> MEVNVKGNYVQVYVMLPLDAVSVNNRFEKGDELRAQLRKLVEAGVDGVMVDVWWGLVEGKGPKAYDWSAYKQLFELVQKAGLKLQAIMSFHQCGGNVGDAVNIPIPQWVRDVGTRDPDIFYTDGHGTRNIEYLTLGVDNQPLFHGRSAVQMYADYMTSFRENMKEFLDAGVIVDIEVGLGPAGEMRYPSYPQSHGWSFPGIGEFICYDKYLQADFKAAAAAVGH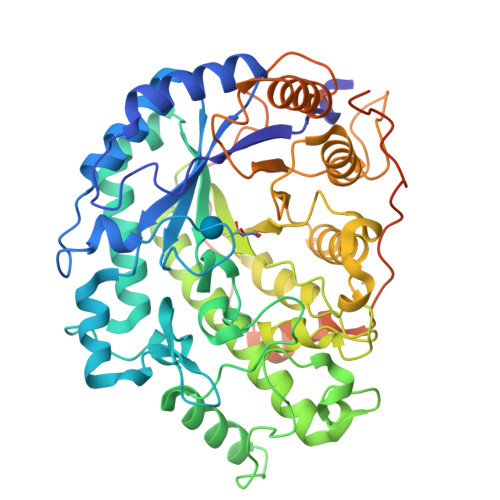PEWEFPNDVGQYNDTPERTQFFRDNGTYLSEKGRFFLAWYSNNLIKHGDRILDEANKVFLGYKVQLAIKISGIHWWYKVPSHAAELTAGYYNLHDRDGYRTIARMLKRHRASINFTCAEMRDSEQSSQAMSAPEELVQQVLSAGWREGLNVACENALPRYDPTAYNTILRNARPHGINQSGPPEHKLFGFTYLRLSNQLVEGQNYVNFKTFVDRMHANLPRDPYVDPMAPLPRSGPEISIEMILQAAQPKLQPFPFQEHTDLPVGPTGGMGGQAEGPTCGMGGQVKGPTGGMGGQAEDPTSGMGGELPATM> MDCSTNISPKQGLDKAKYFSGKWYVTHFLDKDPQVTDQYCSS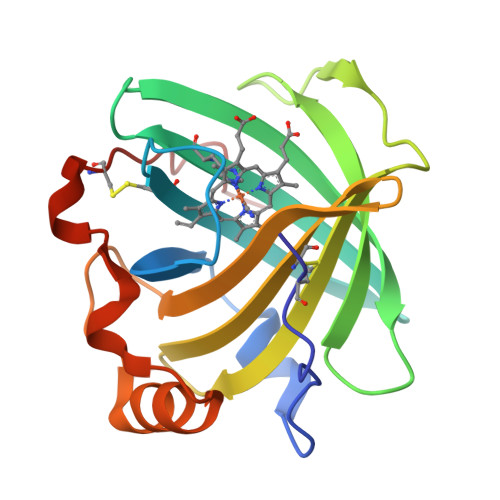FTPRESDGTVKEALYHYNANKKTSFYNIGEGKLESSGLQYTAKYKTVDKKKAVLKEADEKNSYTLTVLEADDSSALVHICLREGSKDLGDLYTVLTHQKDAEPSAKVKSAVTQAGLQLSQFVGTKDLGCQYDDQFTSL(2R)-5-[(acetyloxy)methyl]-2-{(1R)-2-oxo-1-[(thiophen-2-ylacetyl)amino]ethyl}-3,6-dihydro-2H-1,3-thiazine-4-carboxylic acid | C16 H18 N2 O6 S2 | 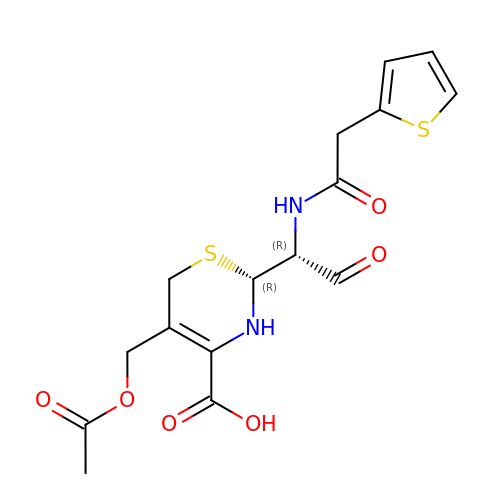MXSQWXIVWHYOCY-IUODEOHRSA-N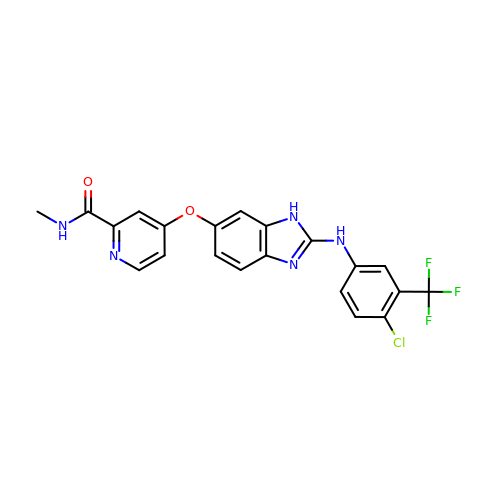4-[[2-[[4-chloro-3-(trifluoromethyl)phenyl]amino]-3H-benzimidazol-5-yl]oxy]-N-methyl-pyridine-2-carboxamide | C21 H15 Cl F3 N5 O2 | ZJLSMLDOCGOURY-UHFFFAOYSA-N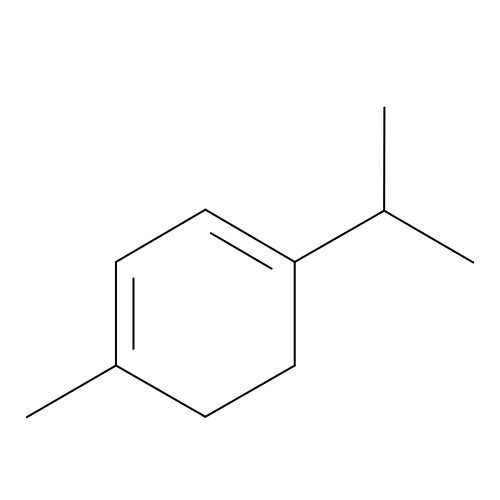1-methyl-4-(propan-2-yl)cyclohexa-1,3-diene | C10 H16 | YHQGMYUVUMAZJR-UHFFFAOYSA-N> GEDKHDIVDGLQLAKQYGHSRQDINIAEYWVSEKLDGIRARWDGTELRTRNNNKIDAPAWFTANWPKATIDGELWIARGQFERTASIVLSKLTSVAPQSVAGSLPRTESTVDAMTATHSLPSKRWAKVRFMAFDMPVAGQSFDSRLNMLNNLKEATPNPTFAVVSQFTLSSVNALEEKLEQVTLSGGEGLMLHHKKAFYHSGRSDKLIKVKQFEDAEAKVLAHFAGKGKFKGMMGSLLVETPAGVQFKLGTGFSEKERRAPPAVGSWVTFKFYGVTKNGKPRFASFLRVRPPSDLPK

DNA ligases catalyze the formation of phosphodiester bonds between adjacent 5′P and 3′OH ends in the backbone of double-stranded DNA and have a conserved core structure comprising the catalytic adenylation (AD) domain and an oligonucleotide-binding (OB) domain joined by a flexible linker region. Catalysis proceeds in a three-step reaction, with step 1 involving nucleophilic attack, by a conserved lysine residue on the α-phosphate of an adenylated cofactor, which can be ATP or NAD+, generating a covalent enzyme-adenylate that is poised to bind the nicked DNA substrate. In step 2, the adenosine monophosphate (AMP) moiety is transferred to the 5′ phosphate of the nicked DNA activating it for attack by the 3′OH in step 3 forming a new phosphodiester bond that seals the break across the DNA backbone. The minimal Lig E-type DNA ligases comprise a clade of phylogenetically distinct ATP-dependent DNA ligases found almost exclusively in proteobacteria.

To further explore the mechanism of Lig E DNA ligases we have carried out site-directed mutagenesis of Psy-Lig and determined the structure of a close homolog from the marine gamma proteobacterium Alteromonas mediterranea Lig E (Ame-Lig) bound to nicked adenylated DNA. The overall structure of the Ame-Lig-DNA complex resolved to 2.3 Å clearly reveals that this Lig E-type ligase binds its substrate without complete encirclement of the DNA duplex. As with other DNA-ligase intermediates, the core catalytic domains of Ame-Lig are oriented to form a C-shaped clamp about the DNA with the nick positioned above the AMP-binding pocket. Inspection of the electron density reveals a phosphodiester bond between the 5′P of the nicked strand and the alpha phosphate of the AMP, indicating that the step two intermediate has been crystalized after transfer of the cofactor from the catalytic lysine K34 to the DNA. DNA encirclement by Ame-Lig encompasses ∼245° of the helix circumference, and the interaction buries 3837 Å2 of contact surface. Continuous electron density is observed for most the protein chain from I7 to R290 with the exception of residues 20–21, and a 26 residue section in the AD domain (S94–S119). The DNA-binding footprint of Ame-Lig is 8 nucleotides (nt29–nt36) on the nicked strand and 12 nucleotides on the complement (nt5–nt16), thus smaller than any previously-described DNA-bound ligase structure. The two terminal base pairs of the nick are distorted into an RNA-like A structure with the sugar moiety adopting a C3′ endo conformation and shortened distances between backbone phosphates, while the remainder of the duplex adopts the preferred DNA-B form. As is the case with other previously-described ligase–DNA intermediates, this distortion is a consequence of two conserved phenylalanines F81 and F283 stacking against the sugars of the 5′PO4 and 3′OH nucleotides.>MASMERFLSVYDEVQAFLLDQLQSKYEIDPNRARYLRIMMDTTCLGGKYFRGMTVVNVAEGFLAVTQHDEATKERILH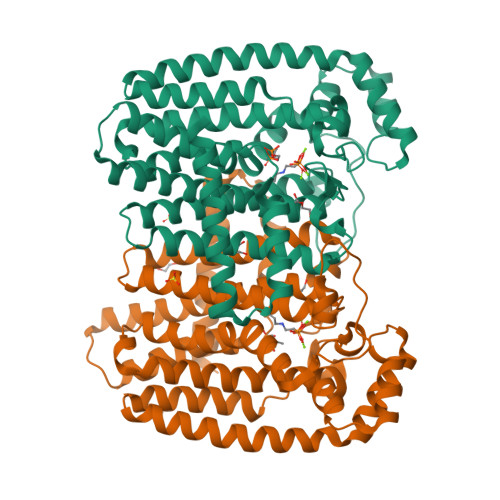DACVGGWMIEFLQAHYLVEDDIMDGSVMRRGKPCWYRFPGVTTQCAINDGIILKSWTQIMAWHYFADRPFLKDLLCLFQKVDYATAVGQMYDVTSMCDSNKLDPEVAQPMTTDFAEFTPAIYKRIVKYKTTFYTYLLPLVMGLFVSEAAASVEMNLVERVAHLIGEYFQVQDDVMDCFTPPEQLGKVGTDIEDAKCSWLAVTFLGKANAAQVAEFKANYGDKDPAKVAVVKRLYSEANLQADFAAYEAEVVREVESLIEQLKVKSPTFAESVAVVWEKTHKRKK[3x]Cholesterol absorption within enterocytes is mediated by Niemann-Pick C1 Like 1 (NPC1L1), a protein primarily expressed in the intestine and the target of the cholesterol absorption inhibitor Ezetimibe. NPC1L1 is a polytopic membrane protein that contains two conserved domains: the sterol sensing domain and the NPC1 domain. The NPC1 domain resides in the amino-terminal extracellular loop and is highly conserved in all NPC1 homologues. NPC1L1 has high sequence homology (∼40%) to lysosomal NPC1, which mediates transport of LDL-derived cholesterol out of lysosomes for subsequent delivery to the endoplasmic reticulum and plasma membrane.

A recombinant form of human NPC1L1(NTD) spanning residues 22–284 was produced in High-5 cells using a baculovirus vector. According to size exclusion chromatography, NPC1L1(NTD) exists as a monomer in solution (data not shown). In the current study, we have determined the crystal structure of NPC1L1(NTD) to 2.8 Å resolution in a cholesterol free, closed form. The structure of NPC1L1(NTD), while sharing the same overall topology as NPC1(NTD), reveals a cholesterol binding pocket that is closed from solvent, suggesting a gating mechanism that relies on the movement of multiple elements around the cholesterol entrance. Comparison to the cholesterol free and bound structures of NPC1(NTD) reveals that NPC1L1(NTD) is in a closed conformation and the sterol binding pocket is occluded from solvent. Comparison of apo-NPC1L1(NTD) to the sterol bound forms of NPC1(NTD) suggests a gating model where multiple movements around the entrance to the sterol binding pocket are required to expand the entrance and allow entry of cholesterol. The cholesterol binding pocket is slightly larger than that of NPC1(NTD), suggesting broader sterol specificity. Residues near the C4 position are smaller in NPC1L1 (PHE35 and LEU216) compared to NPC1 (TRP27 and PHE203), increasing the size of the sterol binding pocket and accommodating C4 substituted sterols such as lanosterol. While the residues near the C4 position are smaller in NPC1L1 compared to NPC1, residues around the isooctyl sidechain are roughly equivalent. The addition of an ethyl group at C24 on β-sitosterol would result in an unfavorable steric clash and we were unable to observe significant competitive binding of β-sitosterol to NPC1L1(NTD).

> GAEPYTTIHQPGYCAFYDECGKNPELSGSLMTLSNVSCLSNTPARKITGDHLILLQKICPRLYTGPNTQACCSAKQLVSLEASLSITKALLTRCPACSDNFVNLHCHNTCSPNQSLFINVTRVAQLGAGQLPAVVAYEAFYQHSFAEQSYDSCSRVRVPAAATLAVGTMCGVYGSALCNAQRWLNFQGDTGNGLAPLDITFHLLEPGQAVGSGIQPLNEGVARCNESQGDDVATCSCQDCAASCPAIARPQALDSTFYLGQMPGS>[6x]GARASVLSGGELDKWEKIRLRPGG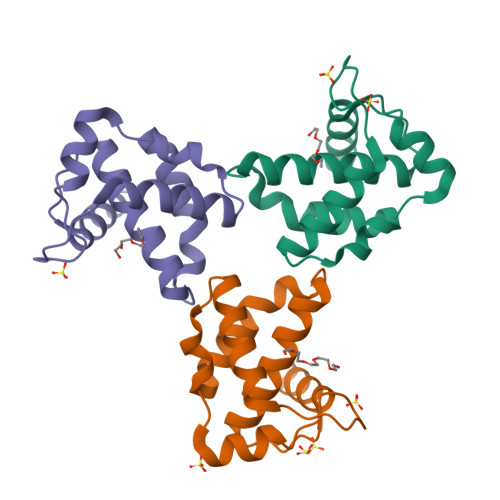KKQYKLKHIVWASRELERFAVNPGLLETSEGCRQILGRLQPSLQTGSEELRSLYNTIAVLYCVHQRIDVKDTKEALDKIEEEQNKSKKKAQQAAADTGNNSQVSQNYHHHHHH>[2x]HHHHHHGSMQILLANPRGFCAGVDRAISIVENALAIYGAPIYVRHEVVHNRYVVDSLRERGAIFIEQISEVPDGAILIFSAHGVSQAVRNEAKSRDLTVFDATCPLVTKVHMEVARASRRGEESILIGHAGHPEVEGTMGQYSNPEGGMYLVES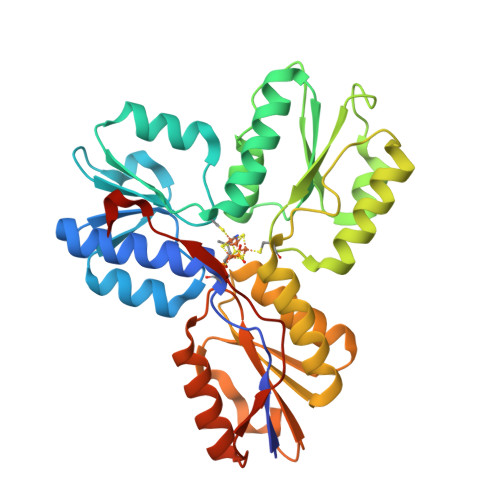PDDVWKLTVKNEEKLSFMTQTTLSVDDTSDVIDALRKRFPKIVGPRKDDICYATTNRQEAVRALAEQAEVVLVVGSKNSSNSNRLAELAQRMGKRAFLIDDAKDIQEEWVKEVKCVGVTAGASAPDILVQNVVARLQQLGGGEAIPLEGREENIVFEVPKELRVDIREV> SLGGARRFLCGVVEGFYGRPWVMEQRKELFRRLQKWELNTYLYAPKDDYKHRMFWREMYSVEEAEQLMTLISAAREYEI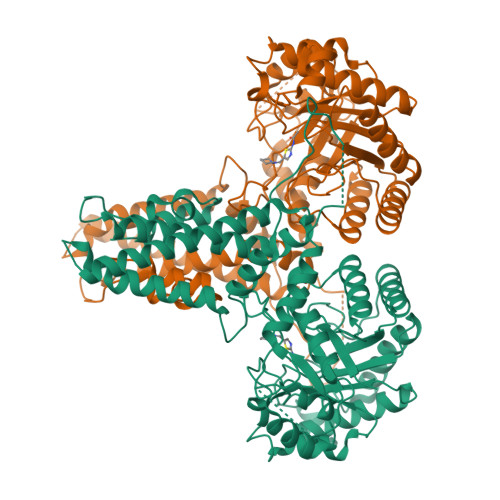EFIYAISPGLDITFSNPKEVSTLKRKLDQVSQFGCRSFALLFDDIDHNMCAADKEVFSSFAHAQVSITNEIYQYLGEPETFLFCPTEYCGTFCYPNVSQSPYLRTVGEKLLPGIEVLWTGPKVVSKEIPVESIEEVSKIIKRAPVIWDNIHANDYDQKRLFLGPYKGRSTELIPRLKGVLTNPNCEFEANYVAIHTLATWYKSNMNGVRKDVVMTDSEDSTVSIQIKLENEGSDEDIETDVLYSPQMALKLALTEWLQEFGVPHQYSSRQVAHSGAKASVVDPGPNEKPLYTAEPVTLEDLQLLADLFYLPYEHGPKGAQMLREFQWLRANSSVVSVNSKGKDSEKIEEWRSRAAKFEEMCGLVMGMFTRLSNCANRTILYDMYSYVWDIKSIMSMVKSFVQWLGERSHSSAQFLIGDQEPWAFRGGLAGEFQRLLPIDGANDLFFQPPPLTPTSK> MGSSHHHHHHSQDPNSMGKLTLLLLAILVWLQYSLWFGKNGIHDYTRVNDDVAAQQATNAKLKARNDQLFAEIDHLNGGQEALEERARNELSMTRPGETFYRLVPDASKRAQSAGQNNR;> MISRVTEALSKVKGSMGSHERHALPGVIGDDLLRFGKLPLCLFICIILTAVTVVTTAHHTRLLTAQREQLVLERDALDIEWRNLILEENALGDHSRVERIATEKLQMQHVDPSQENIVVQK;> MSQAALNTRNSEEEVSSRRNNGTRLAGILFLLTVLTTVLVSGWVVLGWMEDAQRLPLSKLVLTGERHYTRNDDIRQSILALGEPGTFMTQDVNIIQTQIEQRLPWIKQVSVRKQWPDELKIHLVEYVPIARWNDQHMVDAEGNTFSVPPERTSKQVLPMLYGPEGSANEVLQGYREMGQMLAKDRFTLKEAAMTARRSWQLTLNNDIKLNLGRGDTMKRLARFVELYPVLQQQAQTDGKRISYVDLRYDSGAAVGWAPLPPEESTQQQNQAQAEQQ

The essential membrane protein complex of FtsB, FtsL and FtsQ (FtsBLQ) is at the heart of the divisome assembly cascade in Escherichia coli. This complex regulates the transglycosylation and transpeptidation activities of the FtsW-FtsI complex and PBP1b via coordination with FtsN, the trigger for the onset of constriction. A core complex at the heart of this machinery is composed of three type-II bitopic membrane proteins, the Filamentous temperature-sensitive proteins B, L and Q (FtsB, FtsL, FtsQ). For a long time, the FtsBLQ complex was believed to act as a non-enzymatic scaffold for the assembly of the divisome, but recent studies revealed it to be a positive regulator of the FtsWI complex and a negative regulator of the bi-functional PG synthase PBP1b.

Finally, it is important to note that two CCD residues, FtsBE56 and FtsBD59, are buried in the FtsB-FtsQ interface, especially for the interaction hot-spot FtsBE56 which has an accessible surface area (ASA) of only 3.8 Å², about 2% in ASA ratio. We found that the mutations of FtsBE56A or FtsBD59H did not affect the complex formation on SEC or the overall structure (RMSD ~ 0.45 Å from the wild type), and a mechanistic explanation is lacking for their apparent function in promoting cell constriction. Crystal structures of FtsBE56ALQ and FtsBD59HLQ mutant complexes were solved, revealing a displacement of the FtsB α2-α3 linker for ~2–4 Å. While the overall structures remained almost the same probably due to the stabilization of crystal packing, the coiled coil might be more prone to move and this tendency could be transferred to their C-terminal linkers. When no such external force existed in solution, we observed a dramatic reduction of the higher-order oligomer band on native PAGE of the FtsBE56A and FtsBD59H mutants, indicating that the inter-oligomer contact may be affected by a potential allosteric change. Herein, unless the FtsBLQ complex adopts a different conformation in vivo which exposes FtsBE56 and FtsBD59 for direct interactions with PBP1b or FtsWI, the only other possibility for these residues to affect cell division should lie in the FtsB-FtsQ interface, which connects the coiled coil to FtsQ. Mutations that disrupt this connection may detach the coiled coil from FtsQ, and the coiled coil may move accordingly to fit the short TM domains of FtsBL in a less tilted orientation in the membrane. Although no conclusion could yet be made, the CCD residues, FtsBE56 and FtsBD59, are likely to function as a negative regulatory element to allosterically prevent any undesired movement in the balanced interplay between FtsBLQ and the PG synthases. Mutations of FtsBE56 and FtsBD59, on the other hand, may induce a conformational change of the coiled coil to further enhance the activation of FtsWI, impair the inhibition of PBP1b and promote constriction.> MKKILNSLFSITLVMLVPFKVMASWYEVTGVATIVSSEETARLHALEDALFKAVNFSGADIGSISNLMPLLEESRNEYQFTNHEVRYILVESERKRRGKVEVKIRVDIYPSATGCHTDQYKKTILVGNIEVASPQQAVMGQIYQVGDDFSRVVNRQLDQTSRSFVSVGTTDYSISSNYPARTQMIAQDNGAQYIIGGVITDLTATVESQLLQDDIINRQFALEMKVFDGKTGHEV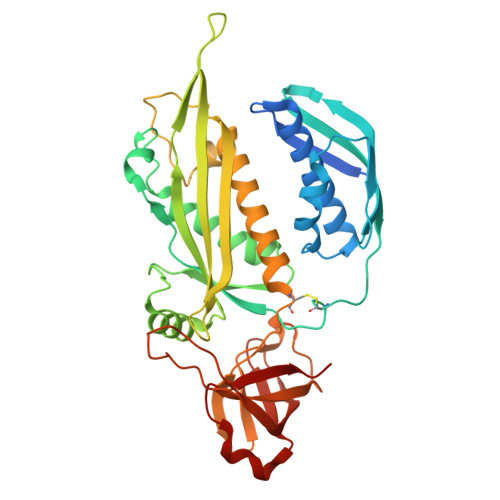FNKAYREVARWPFAKTSQVDTRSARFWASTYGEMMLRVSRNIMLDLESELSCKITLPEVVAVFGNTVTMDLGRMHGVKEGDKLQLWHTASFIDQNGLPRNKVSQSEITLTVSRIYEHEAELTIDQPNLASSVQIGDVMNKIL N-{(4M)-4-[5-(aminomethyl)thiophen-2-yl]quinolin-8-yl}-4-[(propan-2-yl)oxy]benzamide 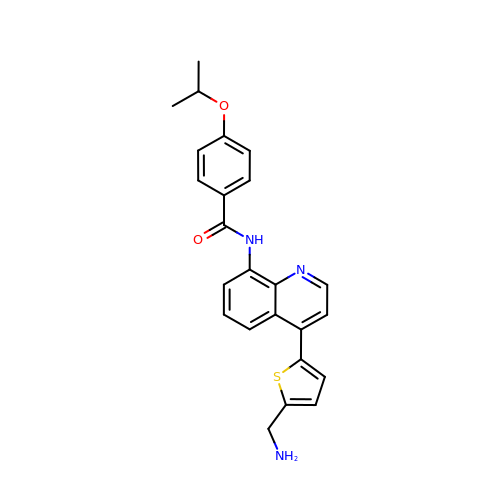| C24 H23 N3 O2 S | ZHPRIQJGWCNUFC-UHFFFAOYSA-N>[2x]AEAGITGTWYNQLGSTFIVTAGADGALTGTYESAVGNAESRYVLTGRYDSAPATDGSGTALGW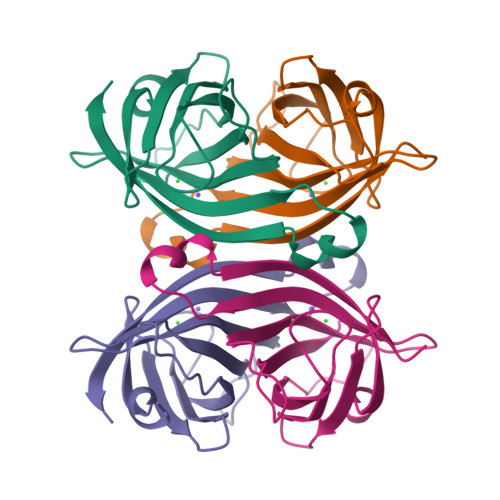TVAWKNNYRNAHSATTWSGQYVGGAEARINTQWLLTSGTTEANAWKSTLVGHDTFTKVKP> GSMDSSPNEFLNKVIGKKVLIRLSSGVDY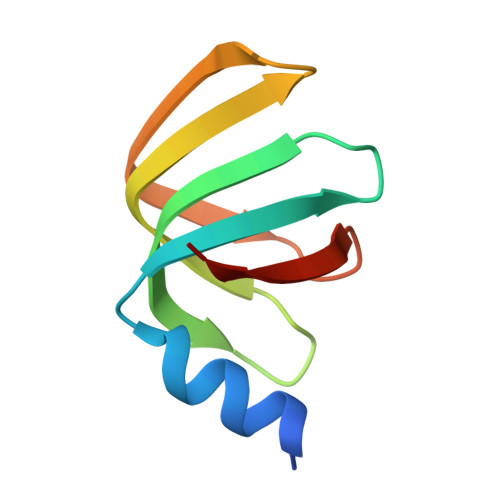KGILSCLDGYMNLALERTEEYVNGKKTNVYGDAFIRGNNVLYVSALDD DIPHENYLACETIC ACID | C14 H12 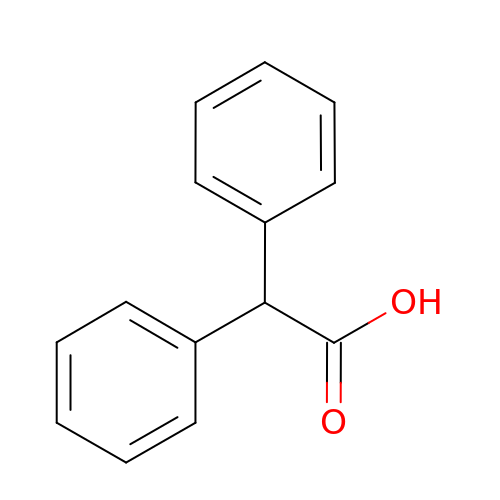O2 | PYHXGXCGESYPCW-UHFFFAOYSA-N>[2x]MVEKGKMVKISYDGYVDGKLFDTTNEELAKKEGIYNPAMIYGPVAIFAGEGQVLPGLDEAILEMDVGEEREVVLPPEKAFGKRDPSKIKLIPLSEFTKRGI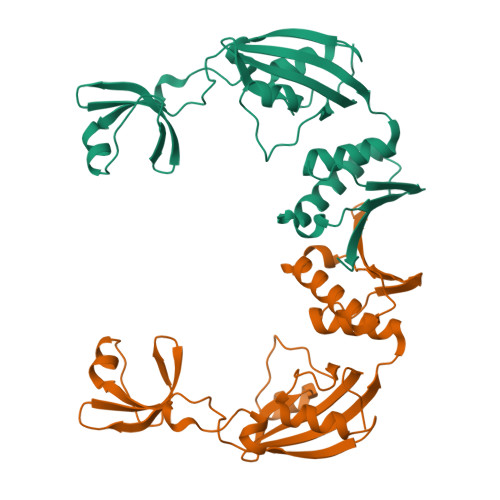KPIKGLTITIDGIPGKIVSINSGRVLVDFNHELAGKEVKYRIKIEEVVDDKKNIVKEIVKMYVPRLSDVKVTIRNGTVKIELPEFAPFIPNIQTAKMAIANEILKRLEDAEKVSFVETFERKKETKEENK>FEDRDPTQFEERHLKFLQQLGKGNFGSVEMCRYDPLQDNTGEVVAVKKLQHSTEEHLRDFEREIEILKSLQHDNIVKYKGVCYSAGRRNLRLIMEYLPYGSLRDYLQKHKERIDHKKLLQYTSQICKGMEYLGTKRYIHRDLATRNILVENENRVKIGDFGLTKVLPQDKEYYKVKEPGESPIFWYAPESLTESKFSVASDVWSFGVVLYELFTYIEKSKSPPVEFMRMIGNDKQGQMIVFHLIELLKSNGRLPRPEGCPDEIYVIMTECWNNNVSQRPSFRDLSLRVDQIRDSIAA[4x];>[4x]QGAHDLKTFSSKSEYQLVVNAVRKLQESGFYWSAVTGGEANLLLSAEPAGTFLIRDSSDQRHFFTLSVKTQSGTKNLRIQCE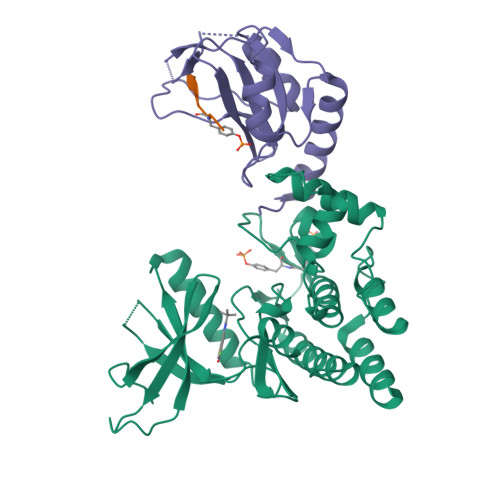GGSFSLQSDPRSTQPVPRFDCVLKLVHHYMGSGSGSGSRAYYIYSGGEKIPLVLSRPLSSN;>STASTVEYSTVVHSG[4x]>[4x]MEIAFLLNGETRRVRIEDPTQSLLEWLRAEGLTGTKEGCNEGDCGACTVMIRDAAGSRAVNACLMMLPQIAGKALRTIEGIAAPDGRLHPVQQAMIDHHGSQCGFCTPGFIVSMAAAHDRDRKDYDDLLAGNLCRCTGYAPILRAAEAAAGEPPADWLQADAAFTLAQLSSGVRGQTAPAFLPETSDALADWYLAHPEATLIAGGTDVSLWVTKALRDLPEVAFLSHCKDLAQIRETPDGYGIGAGVTIAALRAFAEGPHPALAGLLRRFASEQVRQVATIGGNIANGSPIGDGPPALIAMGASLTLRRGQERRRMPLEDFFLEYRKQDRRPGEFVESVTLPKSAPGLRCYKLSKRFDQDISAVCGCLNLTLKGSKIETARIAFGGMAGVPK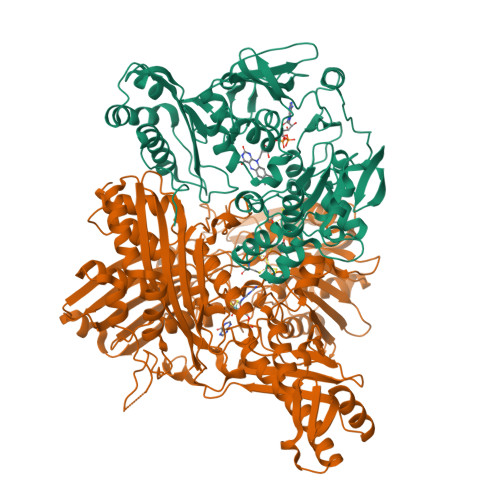RAAAFEAALIGQDFREDTIAAALPLLAQDFTPLSDMRASAAYRMNAAQAMALRYVRELSGEAVAVLEVMP;>MSVGKPLPHDSARAHVTGQARYLDDLPCPANTLHLAFGLSTEASAAITGLDLEPVRESPGVIAVFTAADLPHDNDASPAPSPEPVLATGEVHFVGQPIFLVAATSHRAARIAARKARITYAPRPAILTLDQALAADSRFEGGPVIWARGDVETALAGAAHLAEGCFEIGGQEHFYLEGQAALALPAEGGVVIHCSSQHPSEIQHKVAHALGLAFHDVRVEMRRMGGGFGGKQSQGNHLAIACAVAARATGRPCKMRYDRDDDMVITGKRHDFRIRYRIGADASGKLLGADFVHLARCGWSADLSLPVCDRAMLHADGSYFVPALRIESHRLRTNTQSNTAFRGFGGPQGALGMERAIEHLARGMGRDPAELRALNFYDPPERGGLSAPPSPPEPIATKKTQTTHYGQEVADCVLGELVTRLQKSANFTTRRAEIAAWNSTNRTLARGIALSPVKFGISFTLTHLNQAGALVQIYTDGSVALNHGGTEMGQGLHAKMVQVAAAVLGIDPVQVRITATDTSKVPNTSATAASSGADMNGMAVKDACETLRGRLAGFVAAREGCAARDVIFDAGQVQASGKSWRFAEIVAAAYMARISLSATGFYATPKLSWDRLRGQGRPFLYFAYGAAITEVVIDRLTGENRILRTDILHDAGASLNPALDIGQIEGAYVQGAGWLTTEELVWDHCGRLMTHAPSTYKIPAFSDRPRIFNVALWDQPNREETIFRSKAVGEPPFLLGISAFLALHDACAACGPHWPDLQAPATPEAVLAAVRRAEGRA[4x]>GHPETLVKVKDAEDQLGARVGYIELDLNSGKILESFRPEERFPMMSTFKVLLCGAVLSRVDAGQEQLGRRIHYSQNDLVEYSPVTEKHLTDGMTVRELCSAAITMSDNTAANLLLTTIGGPKELTAFLHNMGDHVTRLDRWEPELNEAIPNDERDTTTPAAMATTLRKLLTGELLTLASRQQLIDWMEADKVAGPLLRSALPAGWFIA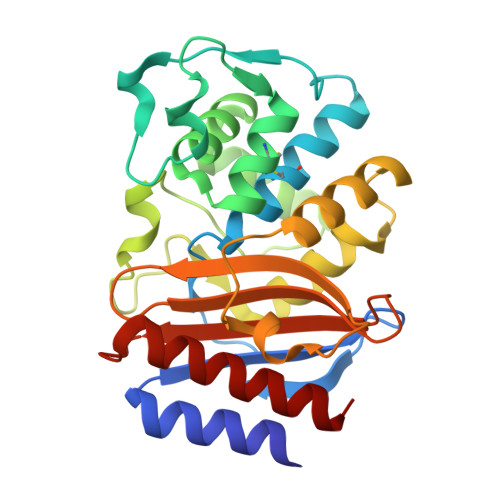DKSGYGERGSRGIIAALGPDGKPSRIVVIYTTGSQATMDERNRQIAEIGASLIKHW[4x]> MSSPSKPTSPFVDDIEHESGSASNGLSSMSPFDDSFQFEKPSSAHGNIEVAKTGGSVLKRQSKPMKDISTPDLSKVTFDGIDDYSNDNDINDDDELNGKKTEIHEHENEVDDDLHSFQATPMPNTGGFEDVELDNNEGSNNDSQADHKLKRVRFGTRRNKSGRIDINRSKTLKWAKKNFHNAIDEFSTKEDSLENS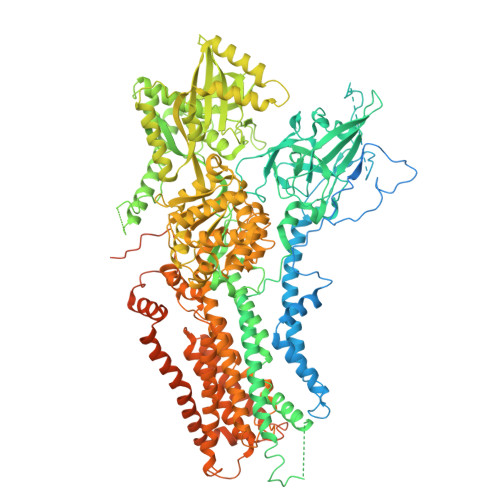ALQNRSDELRTVYYNLPLPEDMLDEDGLPLAVYPRNKIRTTKYTPLTFFPKNILFQFHNFANIYFLILLILGAFQIFGVTNPGFASVPLIVIVIITAIKDGIEDSRRTVLDLEVNNTRTHILSGVKNENVAVDNVSLWRRFKKANTRALIKIFEYFSENLTAAGREKKLQKKREELRRKRNSRSFGPRGSLDSIGSYRMSADFGRPSLDYENLNQTMSQANRYNDGENLVDRTLQPNPECRFAKDYWKNVKVGDIVRVHNNDEIPADMILLSTSDVDGACYVETKNLDGETNLKVRQSLKCSKIIKSSRDITRTKFWVESEGPHANLYSYQGNFKWQDTQNGNIRNEPVNINNLLLRGCTLRNTKWAMGMVIFTGDDTKIMINAGVTPTKKSRISRELNFSVILNFVLLFILCFTAGIVNGVYYKQKPRSRDYFEFGTIGGSASTNGFVSFWVAVILYQSLVPISLYISVEIIKTAQAIFIYTDVLLYNAKLDYPCTPKSWNISDDLGQIEYIFSDKTGTLTQNVMEFKKCTINGVSYGRAYTEALAGLRKRQGVDVESEGRREKEEIAKDRETMIDELRSMSDNTQFCPEDLTFVSKEIVEDLKGSSGDHQQKCCEHFLLALALCHSVLVEPNKDDPKKLDIKAQSPDESALVSTARQLGYSFVGSSKSGLIVEIQGVQKEFQVLNVLEFNSSRKRMSCIIKIPGSTPKDEPKALLICKGADSVIYSRLDRTQNDATLLEKTALHLEEYATEGLRTLCLAQRELTWSEYERWVKTYDVAAASVTNREEELDKVTDVIERELILLGGTAIEDRLQDGVPDSIALLAEAGIKLWVLTGDKVETAINIGFSCNVLNNDMELLVVKASGEDVEEFGSDPIQVVNNLVTKYLREKFGMSGSEEELKEAKREHGLPQGNFAVIIDGDALKVALNGEEMRRKFLLLCKNCKAVLCCRVSPAQKAAVVKLVKKTLDVMTLAIGDGSNDVAMIQSADVGVGIAGEEGRQAVMCSDYAIGQFRYVTRLVLVHGKWCYKRLAEMIPQFFYKNVIFTLSLFWYGIYNNFDGSYLFEYTYLTFYNLAFTSVPVILLAVLDQDVSDTVSMLVPQLYRVGILRKEWNQTKFLWYMLDGVYQSVICFFFPYLAYHKNMVVTENGLGLDHRYFVGVFVTAIAVTSCNFYVFMEQYRWDWFCGLFICLSLAVFYGWTGIWTSSSSSNEFYKGAARVFAQPAYWAVLFVGVLFCLLPRFTIDCIRKIFYPKDIEIVREMWLRGDFDLYPQGYDPTDPSRPRINEIRPLTDFKEPISLDTHFDGVSHSQETIVTEEIPMSILNGEQGSRKGYRVSTTLERRDQLSPVTTTNNLPRRSMASARGNKLRTSLDRTREEMLANHQLDTRYSVERARASLDLPGINHAETLLSQRSRDR> GSSGSSGWVAFDKQVLSFDAYLEEEVLDKSQTNYRIRYYKIYFYPEDDTIQVNEPEVKNSGLLQGTSIRRHRITLP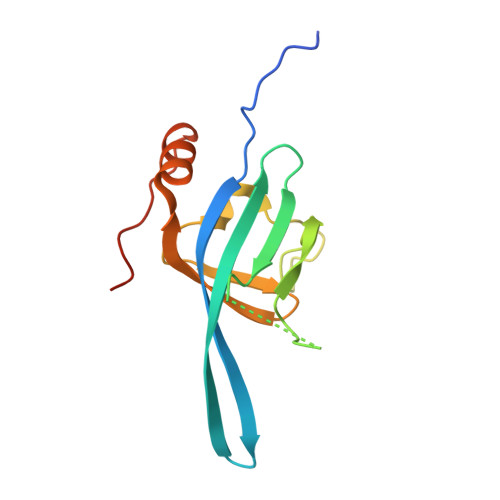PPDEDQFYTVYHFNVGTEVVFYGRTFKIYDCDAFTRNFLRKMGVKVNPPVQSGPSSG> LRAVPGGSSPAWTQCQQLSQKLCTLAWSAHPLVGHMDLREEGDEETTNDVPHIQCGDGCDPQGL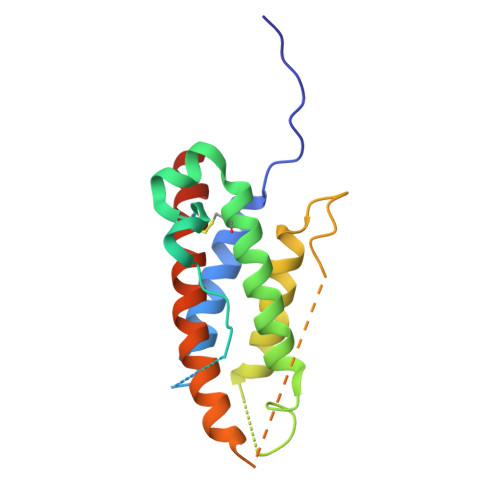RDNSQFCLQRIHQGLIFYEKLLGSDIFTGEPSLLPDSPVGQLHASLLGLSQLLQPEGHHWETQQIPSLSPSQPWQRLLLRFKILRSLQAFVAVAARVFAHGAATLSPHHHHHH>SSSSTASASAKKIIVKHVTVIGGGLMGAGIAQVAAATGHTVVLVDQTEDILAKSKKGIEESLRKVAKKKFAENPKAGDEFVEKTLSTIATSTDAASVVHSTDLVVEAIVQNLKVKNELFKRLDKFAAEHTIFASNTSSLQITSIANATTRQDRFAGLHFFNPVPVMKLVEVIKTPMTSQKTFESLVDFSKALGKHPVSCKDTPGFIVNRLLVPYLMEAIRLYERGDASKEDIDTAMKLGAGYPMGPFELLDYVGLDTTKFIVDGWHEMDAENPLHQPSPSLNKLVAENKFGKKTGEGFYK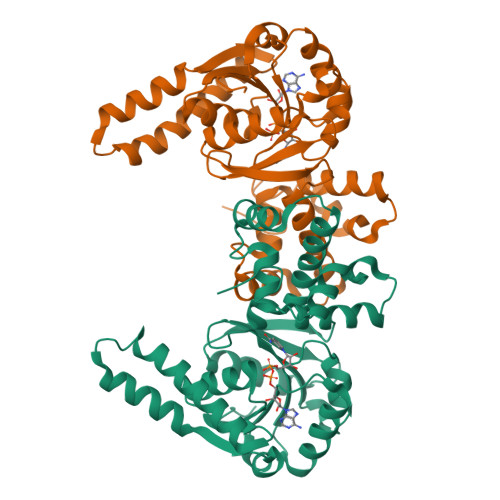YK[2x]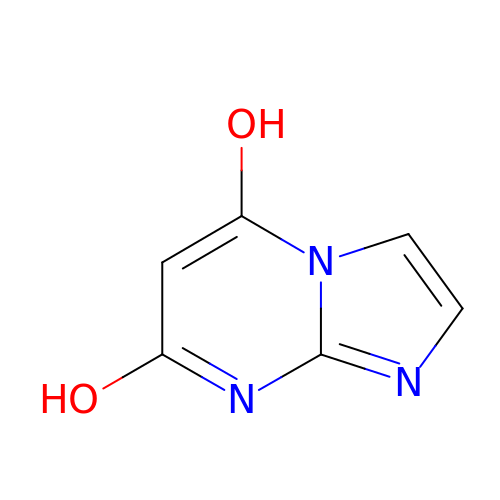(4S)-imidazo[1,2-a]pyrimidine-5,7-diol | C6 H5 N3 O2 | BELWUABPSOOYPK-UHFFFAOYSA-N>[2x]SYADTF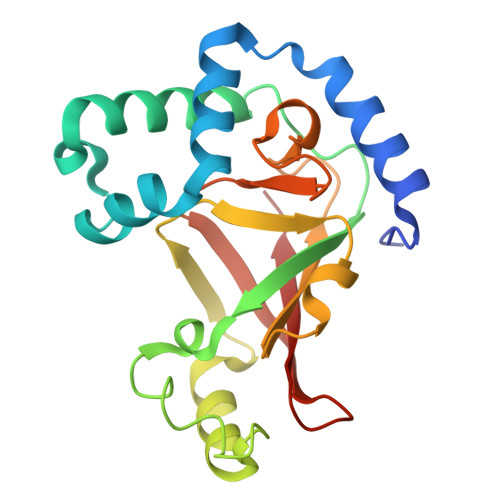TEFTNVEEAKKWGNAQYKKYGLSKPEQEAIKFYTRDASKINGPLRANQGNENGLPADILQKVKLIDQSFSKMKMPQNIILFRGDDPAYLGPEFQDKILNKDGTINKTVFEQVKAKFLKKDRTEYGYISTSLMSAQFGGRPIVTKFKVTNGSKGGYIDPISYFPGQLEVLLPRNNSYYISDMQISPNNRQIMITAMIFK[(2R,3S,4R,5R)-5-(6-amino-9H-purin-9-yl)-3,4-dihydroxyoxolan-2-yl]methyl 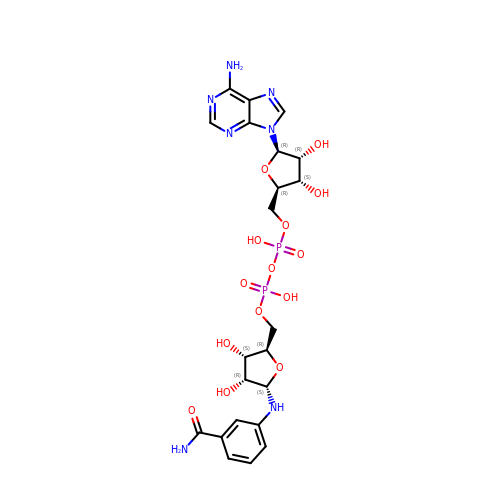[(2R,3S,4R,5S)-5-(3-carbamoylanilino)-3,4-dihydroxyoxolan-2-yl]methyl dihydrogen diphosphate (non-preferred name) | C22 H29 N7 O14 P2 | OJEGJAIQKNCBOQ-ZLPBMXMUSA-N> MVPISPIETVPVKLKPGMDGPKVKQWPLTEEKIKALVEICTEMEKEGKISKIGPENPYNTPVFAIKKKDSTKWRKLVDFRELNKRTQDFWEVQLGIPHPAGLKQKKSVTVLDVSAAFYSVPLDKDFRKYTAFTIPSINNETPGIRYQYNVLPMGWKGSPALLQSSMTKILEPFRKQNPDIVIYQYMDDLYVGSDLEIGQHRTKIEELRQHLLRWGFTTPDKKHQKEPPFLWMGYELHPDKWTVQPIVLPEKDSWTVNDIQKLVGKLNWASQIYAGIKVRQLSKLLRGTKALTEVVPLTEEAELELAENREILKE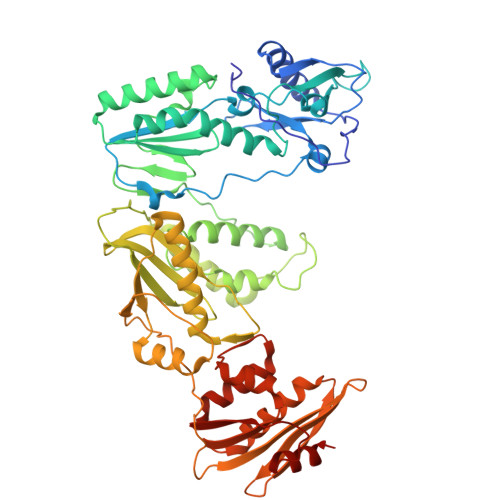PVHGVYYDPSKDLIAEIQKQGQGQWTYQIYQEPFKNLKTGKYARMKGAHTNDVKQLTEAVQKIATESIVIWGKTPKFKLPIQKETWEAWWTEYWQATWIPEWEFVNTPPLVKLWYQLEKEPIIGAETFYVDGAANRETKLGKAGYVTDRGRQKVVPLTDTTNQKTELQAIHLALQDSGLEVNIVTDSQYALGIIQAQPDKSESELVSQIIEQLIKKEKVYLAWVPAHKGIGGNEQVDKLVSAG> MVSQEELIREARQNGMELYPIDKDTYELFFGPQHMATENFSIILKMDGNRVVKAIANPGFLHRGFEKLAEYRPWYTNIALLLRICVPEPDVPEAIYSMAVDEIIGWEVPERAQWIRTLVLEMARVTAYLFWIMGLSFKLGVYTAGQWAAAYRERFMALFEQLTGARVYHIYTIPGGVRRDIPGDKWLRQVRDTVEYLKDKLKDFDNVLFENYITYKRLEGIGVMDKKFALEEGVTGPNLRATGVAYDVRKSDPYLLYPELDFEIPVLKEGDALARVLVRRYELEQDLYIIEQLLDMGPPSGPYKVQDP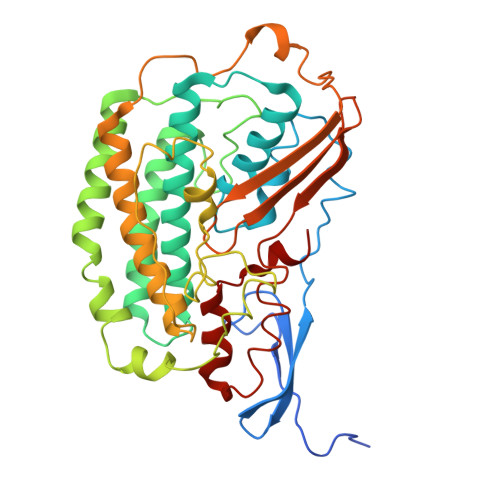KLKNLPRFKVPPGEAFAHVEATKGDFGAYVVSDGGHKPYRVHIRGPSIAHGVRVLEQLLVGARLADVPAILMSLDNCPPDIDR> XXXXXXXXXXXXXXXXXXXXXXXXXXXXXXXXXXXXXXGTVTVRLAASTHAEGTMIADALRRAHLVDGIPWSQMAVIVRSVPRVGTALARALTAAGVPVQDNGTDVPVGRQPAAAALLTVLDVTATGHLDADSAVALLTGPIGRVDPVTLRQLRRALRRADGSQPPRDFGDLLVDAIEREPKGLSAEHARTLRRLRAVLTAARRSDASGADPRYTLWQAWHASGLQRRWLAASERGGSVGAQADRDLDAVTTLFDVADQYVNRTAGASLRGLVDHVTRLGAAVARTEPETAAEAVAVLSVHGALAGEWDFVVIAGVQEGLWPNMIPRGGVLGTQHLVDVLDGVADMTDRTVSTRAPLVAEERRLLMAAMGRARTRVMITAVDSXXXXXXXXXXXXXPPLVAPRVLAPSALVGRLRAVVCAPDGAVDDDARACAAAQLARLAAAGVPGADPSQWHAMTS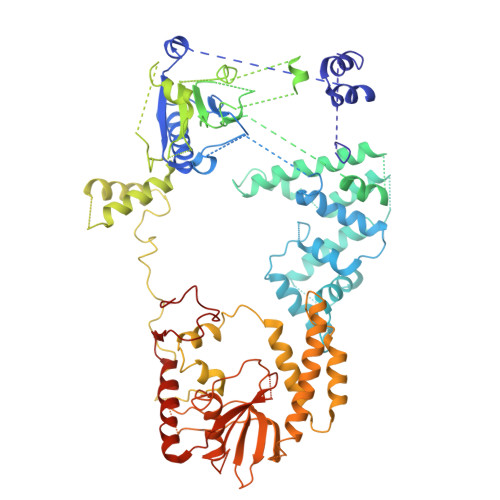LTTEEPLWSEPGHVVTLSPSTLQMLTDCPLRWLLERHGGDDGRDVRSTVGSLVHALVSEPGKTESQLVNELEKVWDDLPYDAKWYSDNELARHRAMLETFTRWREDTRRQLTEVATEIPVEGIVVEPGENTPGVRVRGRLDRLERDEAGRLVVVDLKTGKSPVTKDDAQNHAQLAMYQLAVAAGLLDDGDEPGGGKLVYLGKAGAAGATEREQDPLTPDKRAEWLETVGEAAAATAGPRFVARVNNGCANCPVRSSCPAQANGDRP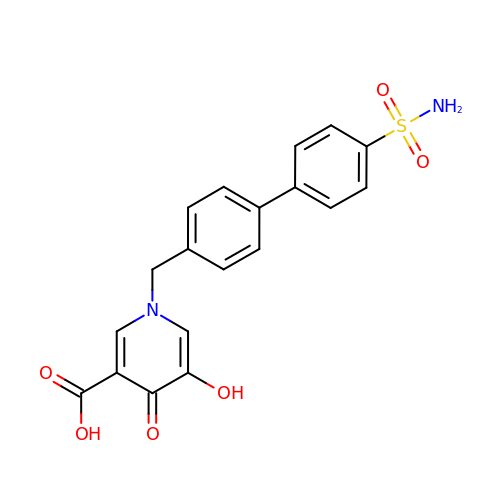5-hydroxy-4-oxo-1-[(4'-sulfamoyl[1,1'-biphenyl]-4-yl)methyl]-1,4-dihydropyridine-3-carboxylic acid | C19 H16 N2 O6 S | ITQGYJSLTCSCLX-UHFFFAOYSA-N> MSRSKRDNNFYSVEIGDSTFTVLKRYQNLKPIGSGAQGIVCAAYDAILERNVAIKKLSRPFQNQTHAKRAYRELVLMKCVNHKNIIGLLNVFTPQKSLEEFQDVYIVMELMDANLCQVIQMELDHERMSYLLYQMLCGIKHLHSAGIIHRDLKPSNIVVKSDCTLKILDFGLARTAGTSFMMTPYVVTRYYRAPEVILGMGYKENVDIWSVGCIMGEMIKGGVLFPGTDHIDQWNKVIEQLGTPSPEFMKKLQPTVRTYVENRPKYAGYSFEKLFPDVLFPADSEHNKLKASQARDLLSKMLVIDASKRISVDEALQHPYINVWYDPSEAEAPPPKIPDKQLDEREHTIEEWKELIYKEVMDLEH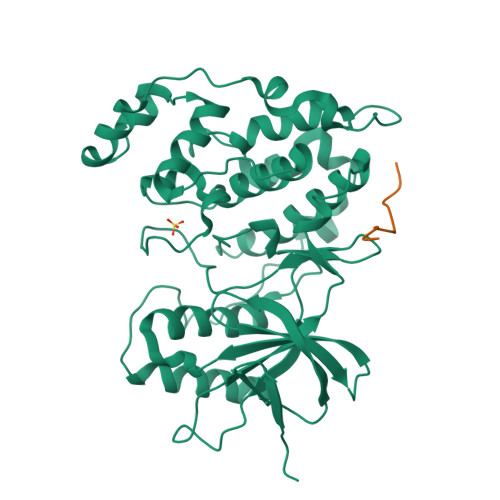HHHHH;> RPKRPTTLNLF[(1S,3S,6S,7S,8R,9S)-6-[(4-methoxyphenyl)methyl]-3-(methylamino)-7-oxidanyl-5-azatricyclo[6.3.1.0^1,5]dodecan-9-yl] dihydrogen phosphate | C20 H31 N2 O6 P | 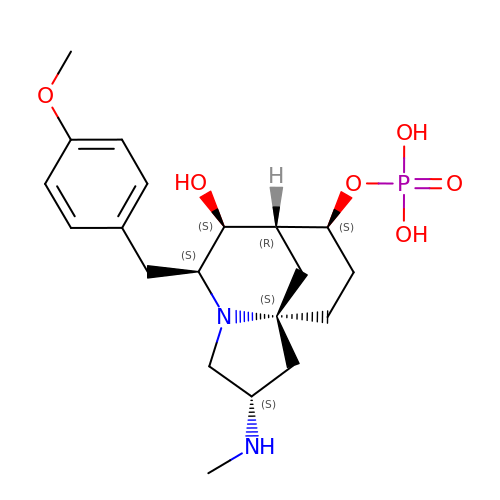CIISYBZFZSWZLX-KKMIJOEASA-N> MQTYLSTKSIEYYLKELKEIFSQIWLKPSEIEKRCEELFKRSKEFDYKRILVSGETDNTTLYVIEDSSKIHVFSPNRDLRENPLLMRWHPSWYEIESKEIYYKCFLSCEELYEHLELPTVTLVNLCVIENFPIPRLNLSTGTLSSYLRKEQLAKVELIDMQVGTTINQIIKNLLDSQPDIIGLSVNFGQKKLAFEILDLIYSHIENGDLSSIITVGNVIPSFSPEQFFERYPSLLICDKE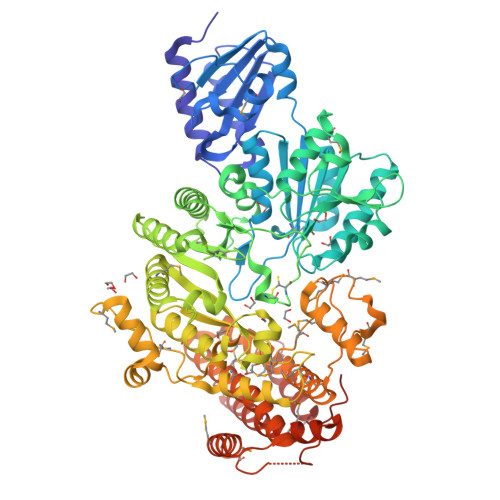GEYTLRDLIKMLKKELKLDEVNGISYVDESGEVKHNVAETVNFKEEVPTPSLDILGEISKFRGALTLETSRGCDYSRCTFCPRDHKLRSWRPLSVEQTLKQLDDILRAGKHFNIKPHIYMADEEFIGELPNGTEAQRIIDICEGLLKREEKIKFDFAARADSVYEPKRTKEWNVERLKMWHYCALAGADRIFIGVESGSNQQLKRYGKGTTSEQNIIALRLVSALGINLRIGFIMFDQLMKGLDNLKENLDFLERTDALMKPIDIGDMTYEELYDKLLNDKEFIEKHKTGKPVYTIVSYMLASMEILMNTPYSRMVQLTERKEEVNLIMNDGKPDMNMGRYATSFVDKTNGNLSEACQMWIDSNFGVMYTIKSLHKVANPREKKKLYSYMETHREISHFLLKYLVYNLSPDKESQIILSDFLRMHSMEHILDNSKINVGDGSKENILNVMTNWQLIMEKLLRDVEADLNKGIITDSEDHRLHNTLKRWFSDMGNWSLINAYELN> SQGVIGIFGDYAKAHDLAVGEVSKLVKKALSNEYPQLSFRYRDSIKKTEINEALKKIDPDLGGTLFVSNSSIKPDGGIVEVKDDYGEWRVVLVAEAKHQGKDIINIRNGLLVGKRGDQDLMAAGNAIDRSHKNISE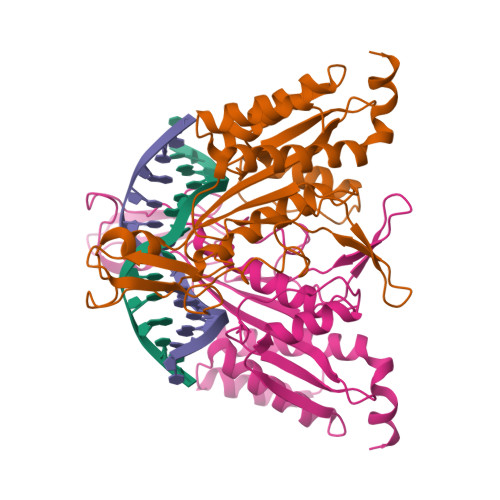IANFMLSESHFPYVLFLEGSNFLTENISITRPDGRVVNLEYNSGILNRLDRLTAANYGMPINSNLCINKFVNHKDKSIMLQAASIYTQGDGREWDSKIMFEIMFDISTTSLRVLGRDLFEQLTSK> MNTKYNKEFLLYLAGFVDGDGSIIAQIEPNASYKFKHRLKLTFKVTQKTQRRWFLDKLVDEIGVGYVRDEGSVSNYILSEIKPLRNFLTQLQPFLKLKQKQANLVLKITEQLPSAKESPDKFLEVCTWVDQIAALNDSKTRKTTSETVRAVLD;> MNTKYNKEFLLYLAGFVDADGSIIAQIAPNQSSKFKHRLKLTFQVTQKTQRRWFLDKLVDEIGVGYVRGSGSVSNYILSEIKPLHNFLTQLQPFLKLKQKQANLVLKIIEQLPSAKESPDKFLEVCTWVDQIAALNDSKTRKTTSETV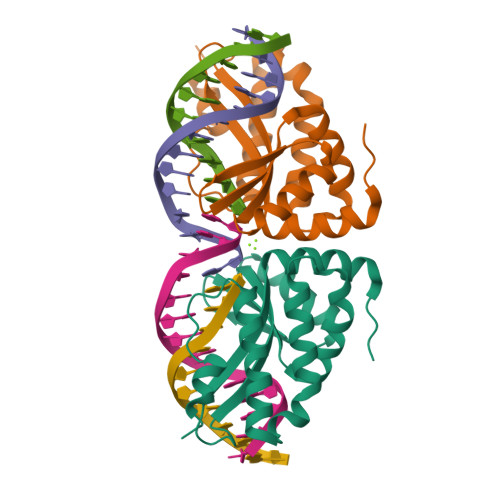RAVLD Bacteriophytochromes (BphPs) are promising design templates for NIR fluorescent proteins. Their covalent association with the linear tetrapyrrole biliverdin IXα (BV) allows BphPs to absorb light in the red and far-red region of the spectrum. While full-length phytochromes are required for biological activity, fluorescence protein development is concentrated to PAS and GAF domains, which together form a chromophore-binding domain (CBD). To increase BphP utility as a fluorophore, residues in this GAF dimer interface have been rationally mutated to create a monomer.

Our motivation in this study has been to explore the effects of a nonpolar substitution of residue 207, which is in closest proximity to the four nitrogen atoms of BV and the ordered pyrrole water found interacting with three of them. In this paper we engineered two DrCBDmon variants containing D207L; DrCBDmon-D207L itself and DrCBDmon-Y263F/D207L (WiPhy2). To gain insight into the fluorescent nature of WiPhy2, a 1.3 Å resolution crystal structure was obtained. There were no significant changes to the overall structure of WiPhy2 compared to DrCBDmon (RMSD 0.82 Å over all 296 shared Cα atoms including mobile loop regions). The BV chromophore is well-ordered with no evidence of a break in electron density for the cysteine connection to the A-ring. The most obvious result from this new structure is the confirmation of our hypothesis: waters are less abundant around the L207 side chain than has been seen in other high-resolution structures containing either Asp or His at this position. For D207L, within 5 Å of any Leu atom there are only four waters, including the pyrrole water with strong interactions to BV nitrogen atoms in A-, B-, and C-rings. Of course, there are no H-bonds from any of these waters to the L207 side chain in WiPhy2. We demonstrate that WiPhy2 has a fluorescence quantum yield of nearly 9% and an excited state lifetime of 780 ps, both ~20% higher than WiPhy, representing the effect of the Leu on the excited state decay of BV in the binding pocket. Indeed, in WiPhy2 Leu at position 207 raises fluorescence quantum yield and lengthens excited state lifetime, maintaining an illumination wavelength of nearly 700 nm while avoiding PPIXα binding or a narrow pH window for efficacy.

> MASMTGGQQMGRGSMSRDPLPFFPPLYLGGPEITTENCEREPIHIPGSIQPHGALLTADGHSGEVLQMSLNAATFLGQEPTVLRGQTLAALLPEQWPALQAALPPGCPDALQYRATLDWPAAGHLSLTVHRVGELLILEFEPTEAWDSTGPHALRNAMSALESAPNLRALAEVATQTVRELTGFDRVMLYKFAPDATGEVIAEARREGLHAFLGHRFPASLIPAQARALYTRHLLRLTADTRAAAVPLDPVLNPQTNAPTPLGGAVLRATSPMHMQFLRNMGVGSSLSVSVVVGGQLWGLIACHHQTPYVLPPDLRTTLEYLGRELSEQVQVKEALEHHHHHH> MSMAEMLRRDEGLRLKVYWDTEGYPTIGIGHLIMKQPVRDMAQI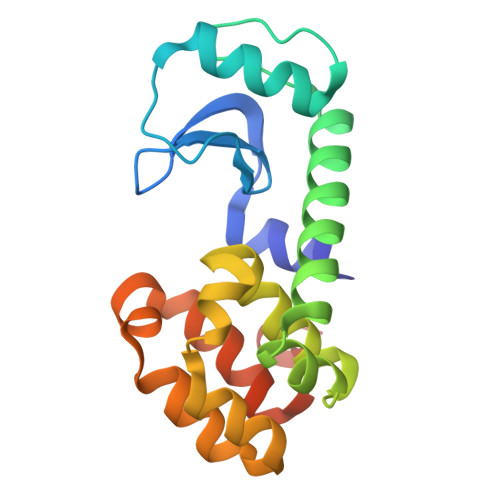NKVLSKQVGREITGNPGSITMEEATTLFERDLADMQRDIKSHSKVGPVWQAVNRSRQMALENMAFQMGVGGVAKFNTMLTAMLAGDWEKAYKAGRDSLWYQQTKGRASRVTMIILTGNLESYGVELEHHHHHH> SYSPT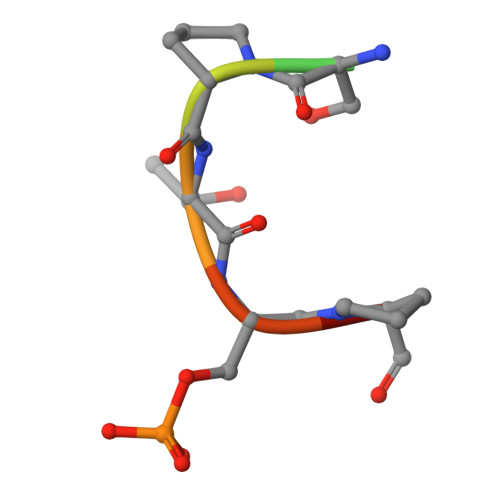SPS>[2x]THTPKLKHLDKLLAHCHRRRYTAKSTIIYAGDRCETLFFIIKGSVTILIEDDDGREMIIGYLNSGDFFGELGLFEKEGSEEERSAWVRAKVE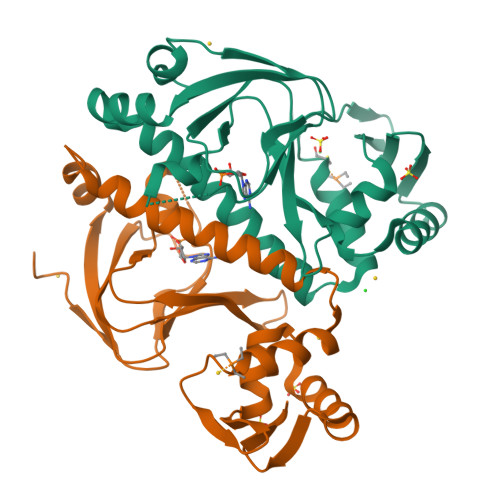CEVAEISYAKFRELSQQDSEILYTLGSQMADRLRKTTRKVGDLAFLDVTGRVARTLLDLCQQPDAMTHPDGMQIKITRQEIGRIVGCSREMVGRVLKSLEEQGLVHVKGKTMVVFGTR> SEDNFARFVCKNNGVLFENQLLQIGLKSEFRQNLGRMFIFYGNKTSTQFLNFTPTLICADDLQTNLNLQTKPV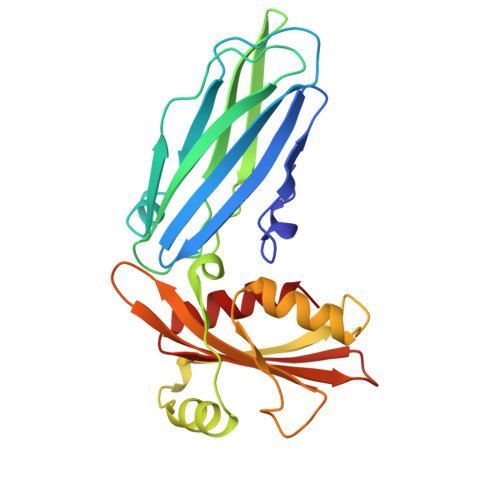DPTVDGGAQVQQVINIECISDFTEAPVLNIQFRYGGTFQNVSVKLPITLNKFFQPTEMASQDFFQRWKQLSNPQQEVQNIFKAKHPMDTEITKAKIIGFGSALLEEVDPNPANFVGAGIIHTKTTQIGCLLRLEPNLQAQMYRLTLRTSKDTVSQRLCELLSEQF2-(1,1-difluoroethyl)-5-methyl-N-[4-(trifluoromethyl)phenyl][1,2,4]triazolo[1,5-a]pyrimidin-7-amine 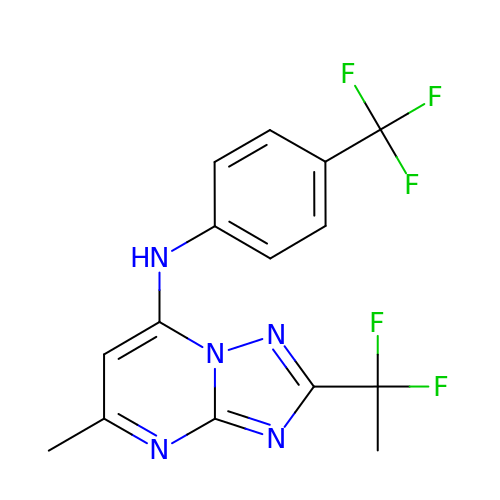| C15 H12 F5 N5 | CUCVTDOXQYMYKL-UHFFFAOYSA-N> QDLTVKMTDLQTGKPVGTIELSQNKYGVVFIPELADLTPGMHGFHIHQNGSCASSEKDGKVVLGGAAGGHYDPEHTNKHGFPWTDDNHKGDLPAL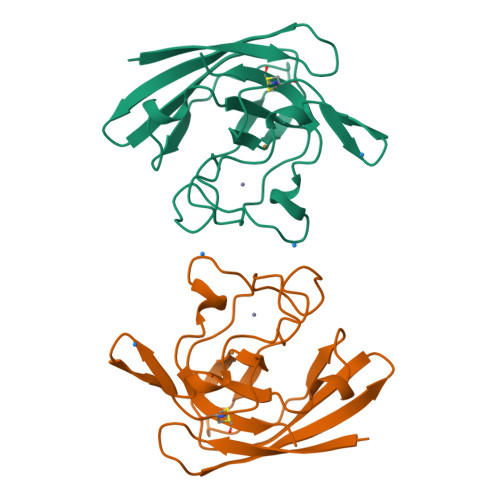FVSANGLATNPVLAPRLTLKELKGHAIMIHAGGDNHSDMPKALGGGGARVACGVIQ> EGLANGEVMSGCHWGVFKARVENGRAVAFEPWDKDPAPSHQLPGVLDSIYSPTRIKYPMVRREFLEKGVNADRSTRGNGDFVRVTWDEALDLVARELKRVQESYGPTGTFGGSYGWKSPGRLHNCQVLMRRALNLAGGFVNSSGDYSTAAAQIIMPHVMGTLEVYEQQTAWPVVVENTDLMVFWAADPMKTNEIGWVIPDHGAYAGMKALKEKGTRVICINPVRTETADYFGADVVSPRPQTDVALMLGMAHTLYSEDLHDKDFLENCTTGFDLFAAYLTGESDGTPKTAEWAAEICGLPAEQIRELARSFVAGRTMLAAGWSIQRMHHGEQAHWMLVTLASMIGQIGLPGGGFGLSYH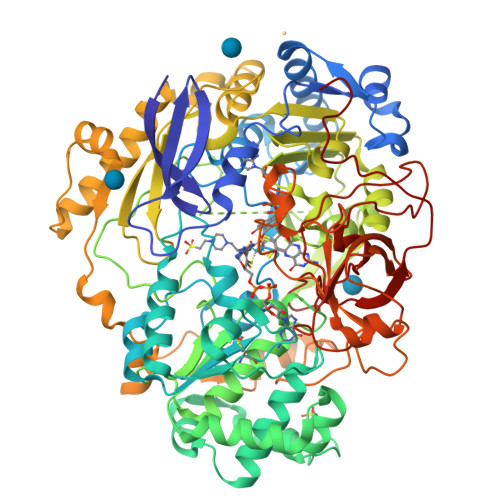YSNGGSPTSDGPALGGISDGGKAVEGAAWLSESGATSIPCARVVDMLLNPGGEFQFNGATATYPDVKLAYWAGGNPFAHHQDRNRMLKAWEKLETFIVQDFQWTATARHADIVLPATTSYERNDIESVGDYSNRAILAMKKVVDPLYEARSDYDIFAALAERLGKGAEFTEGRDEMGWISSFYEAAVKQAEFKNVAMPSFEDFWSEGIVEFPITEGANFVRYADFREDPLFNPLGTPSGLIEIYSKNIEKMGYDDCPAHPTWMEPAERLGGAGAKYPLHVVASHPKSRLHSQLNGTSLRDLYAVAGHEPCLINPADAAARGIADGDVLRVFNDRGQILVGAKVSDAVMPGAIQIYEGGWYDPLDPSEEGTLDKYGDVNVLSLDVGTSKLAQGNCGQTILADVEKYAGAPVTVTVFDTPKGA> MHHHHHHGSLVPRGSMDYKDDDDKENLYFQGSKKIFKPEELRQALMPTLEALYRQDPESLPFRQPVDPQLLGIPDYFDI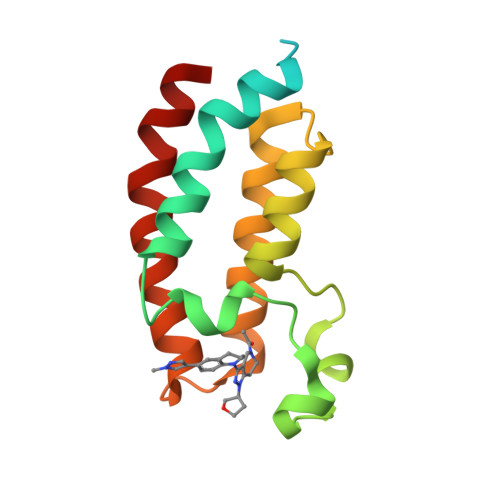VKNPMDLSTIKRKLDTGQYQEPWQYVDDVWLMFNNAWLYNRKTSRVYKFCSKLAEVFEQEIDPVMQSLG> MLSVEKFRVGERVVWIGVIFSGRVQGIAFAFDRGTLMKRIHDLAEHLGKRGVSISLDVQPSDYPEKVFKVLIGELDNASFLRELSFEGVTPFEKKVYEWLTKNVKRGSVITYG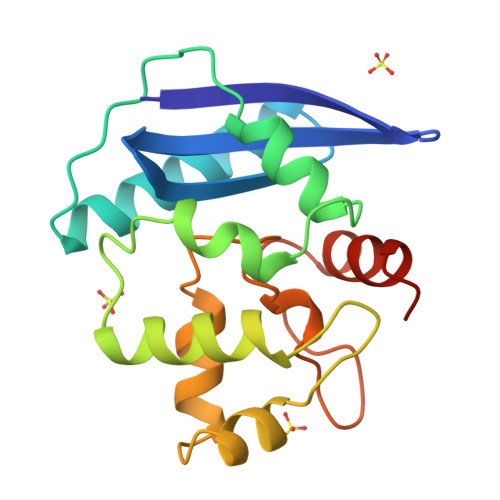DLAKALNTSPRAVGGAMKRNPYPIVVPCHRVVAHDGIGYYSSGIEEKKFLLEIEGVKEWTS> SEEALKWGESLEKLLVHKYGLAVFQAFLRTEFSEENLEFWLACEDFKKVKSQSKMASKAKKIFAEYIA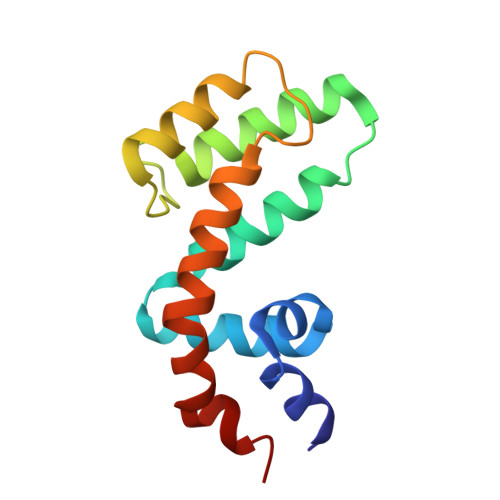IQACKEVNLDSYTREHTKDNLQSVTRGCFDLAQKRIFGLMEKDSYPRFLRSDLYLDLIN> YDGTHCKAPGNCWEPKPGYPDKVAGSKYD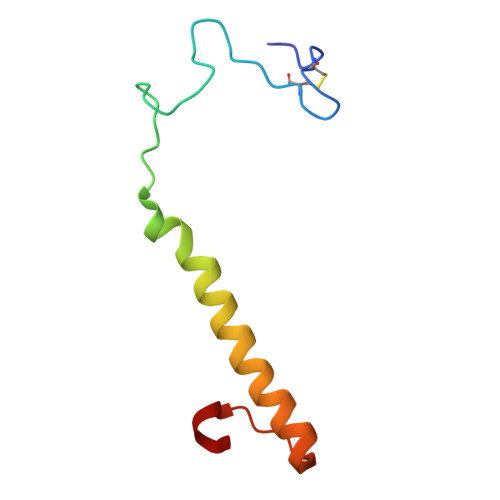PKHDPNELNKQAESIKAMEARNQKRVENYAKTGKFVYKVEDIK> KIRTFGWVQNPGKFENLKRVVQVFDRNSKVHNEVKNIKIPTLVKESKIQKELVAIMNQHDLIYTYKELVGTGTSIRSEAPCDAIIQATIADQGNKKGYIDNWSSDGFLRWAHALGFIEYINKSDSFVITDVGLAYSKSADGSAIEKEILIEAISSYPPAIRILTLLEDGQHLTKFDLGKNLGFSGESGFTSLPEGILLDTLANAMPKDKGEIRNNWEGSSDKYARMIGGWLDKLGLVKQGKKEFIIPTLGKPDNKEFISHAFKITGEGLKVLRRAKGSTKFTRVPKRVYWEMLATNLTDKEYVRTRR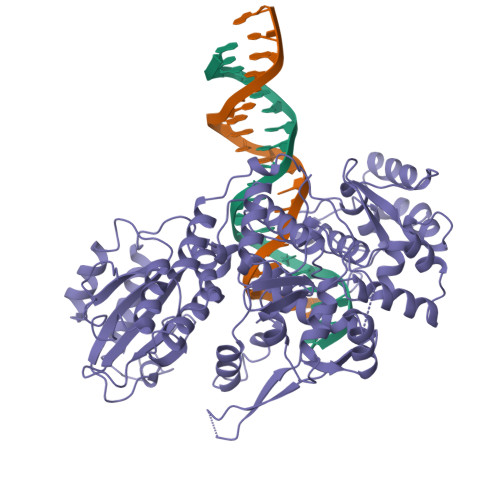ALILEILIKAGSLKIEQIQDNLKKLGFDEVIETIENDIKGLINTGIFIEIKGRFYQLKDHILQFVIPNRGVTKQLVKSELEEKKSELRHKLKYVPHEYIELIEIARNSTQDRILEMKVMEFFMKVYGYRGKHLGGSRKPDGAIYTVGSPIDYGVIVDTKAYSGGYNLPIGQADEMQRYVEENQTRNKHINPNEWWKVYPSSVTEFKFLFVSGHFKGNYKAQLTRLNHITNCNGAVLSVEELLIGGEMIKAGTLTLEEVRRKFNNGEINF Plants have evolved xylanase inhibitor proteins as part of their defense mechanisms against phytopathogens. The rice xylanase inhibitor protein (OsXIP) is structurally similar to GH18 chitinase and homologous to wheat XIP-type inhibitor (XIP-I), which inhibits both GH10 and GH11 xylanases. Various inhibition and interaction analyses showed that OsXIP competitively inhibits the hydrolytic activity of GH11 xylanase RXyn2, but not the activity of GH10 xylanase RXyn1 from Rhizopus oryzae. Although XIP-type inhibitors share significant sequence similarity with GH18 chitinases and adopt a (β/α)8-barrel fold, they are thought to be devoid of chitinase activity because of lack of the catalytic DxDxE motif, which is completely conserved in the catalytic domains of GH18 chitinases.

The OsXIP structure was refined to Rwork/Rfree of 16.6%/17.9% at a resolution of 1.30 Å and shown to adopt a (β/α)8-barrel fold, as observed in family GH18 chitinase structures. Electron density maps of the amino acid residues (Arg155-Val158) consisting of a part of the loop between α4 and β5 (Lα4β5OsXIP) were unobservable in the structure. Although OsXIP shares only 38.2% and 27.6% sequence identity, respectively, with XIP-I and hevamine, a GH18 chitinase from rubber tree Hevea brasiliensis, the main chain structure of OsXIP was closely similar to those of XIP-I and hevamine with RMSDs of 0.85 and 0.77 Å for the corresponding 260 and 253 Cα atoms, respectively. However, in the OsXIP structure, these amino acid residues were substituted, that is, Gln9→Arg18, Asn34→Ser43, Asn45→Asp55, Gly81→Gln85, Ile82→Gly86, Asp125→Phe131, Glu127→Asp133, Tyr183→Phe192, Ala224→Val228, and Trp255→Trp258, respectively, and the substitutions appeared to have caused the protein to lose binding ability of allosamidin. The catalytic signature motif, DxDxE, conserved in GH18 chitinases, was found in center of the groove of hevamine, but not in the structure of OsXIP. In most GH18 chitinases, three disulfide bonds (SS1, SS2, and SS3) are conserved; however, only the two disulfide bonds corresponding to SS1 and SS3 of hevamine are formed in the structure of OsXIP. In particular, the loop between α4 and β5 extruded from the opposite side of the DxDxE catalytic site in hevamine (Lα4β5hev, magenta) consisting of only four amino acid residues (Gly148-Val151), while the corresponding loop in OsXIP (Lα4β5OsXIP) was made of eight amino acid residues (Asp153-Val160) (brown). Although OsXIP possessed Arg155 at the corresponding position, electron density maps of the residues making up a part of Lα4β5OsXIP (Arg155-Val158) were not observed, indicating Lα4β5OsXIP being more conformationally flexible than Lα4β5XIP-I. Furthermore XIP-I has Lys234 in helix α7 (light green), which forms a salt bridge with the acid-base catalyst Glu131 and water-mediated hydrogen bond with the nucleophile Glu239 of XLNC, a GH10 xylanase from A. nidulans, to inhibit its catalytic activity.

> MAVSATSQNTGDTVIIWGRNKDEGSLREACDAGRYTTVIISFLSAFGYIPGTYKLDISGHQVSAVGPDIKYCQSKGKLILLAIGGQGGEYSLPSSQAAVDLHDHLWYSYLGGRRNGVYRPFGDANVNGIDFFIDQGAREHYNELAKMLYDHNKDYRATVGVMVTATTRCGYPDHRLDEALATGLFHRIHVKMFSDGRCPAWSRRQSFEKWAKTYPQSRVLIGVVASPDVDKDAYMPPEALNNLLQFINKQPNFGGVMVWDRFYDKKTGFTAHLHHHHHH> GAMDISQLFHDEVPLF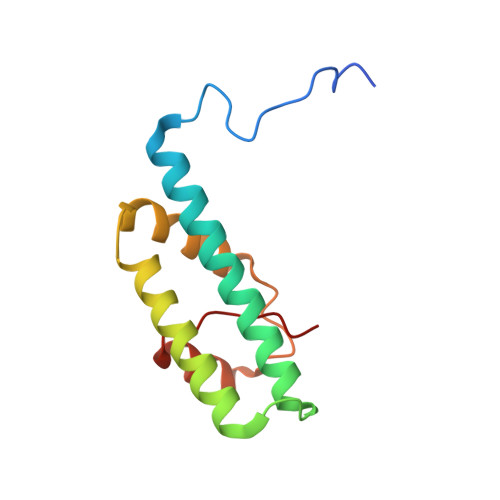DNSITSKDKEVIETLSEIYSIVITLDHVEKAYLKDSIDDTQYTNTVDKLLKQFKVYLNSQNKEEINKHFQSIEAFADTYNITASNAITRLERGIPITAEH>[4x]MAKKTSSKGKLPPVVSSLIPFVGSGLSFAGGPLQYTTDAYKKYGDIFTMKVFGQRLTFLVGPDAHVPFFSQGDAELSQDEPYQFSVPIFGPNVVYGADLAHRNQQLKFIAASLSTKALQSYVPLIVKEAEDFFAKWDKSGTVDIRDALAELIILTASRCLM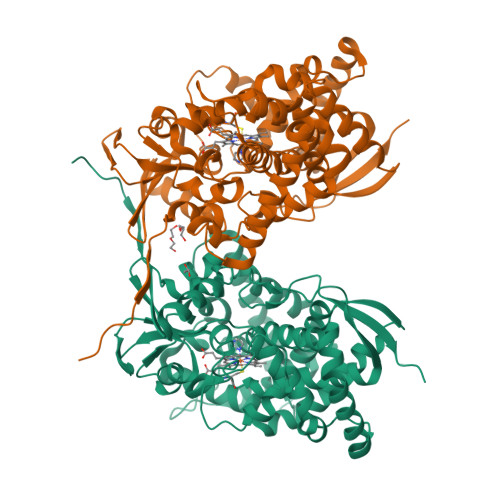GKEIRENLFTEVAKLYQTLDEGLLPISVFFPYLPIPAHKRRDEARLAMVRMFKKIIDERRANPEVKHNDCLQVFMDARYRGEEQALNDEEITGLMIALLFAGQHTSSVTGSWTGLLLFEANNKKKFLPGVLEEQEEIRKEFGDELTMEALNKMDKLHRCVKEALRMYPPLLFVMRKVIKPFSYKDYYVPEGDTVFVSPALSMRVEEVFPNADQYNPERFVEEDKQAQKYRFVGFGAGRHGCMGENFAYLQIKTIWSVLLRNFDIELVGELPKPDYTAMVVGPAHPCLLRYTRKHHHHHH2-azanyl-3-(4-fluorophenyl)carbonyl-indolizine-1-carboxamide | C16 H12 F N3 O2 | 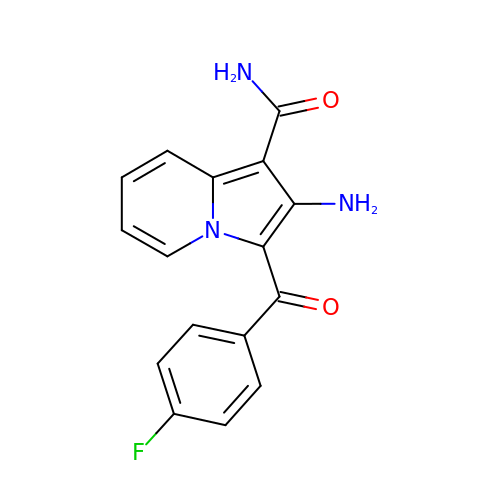ORCDRDYWPJRKDA-UHFFFAOYSA-N> GPVEDAVTAAIGRVADTVGTGPTNSEAIPALTAAETGHTSQVVPGDTMQTRHVKNYHSRSESTVENFLCRSACVYFTEYKNSGSKRYAEWVVTTRQAAQLRRKLEFFTYIRFDLELTFVITSTQQPSTTQNQDAQILTHQIMYVPPGGPVPDKVDSYVWQTSTNPSVFWTEGNAPPRMSIPFLSIGNAYSNFYD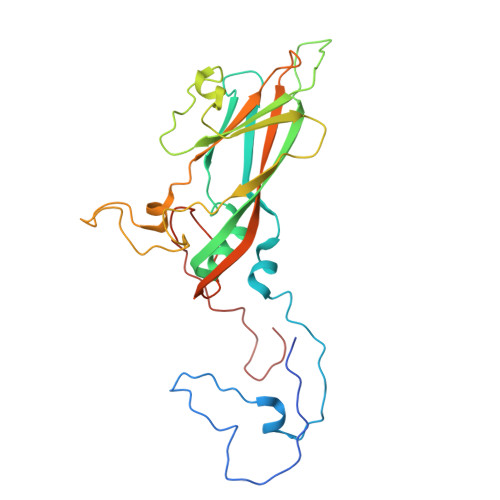GWSDFSRDGVYGINTLNSMGTLYARHVNTGGTGPIKSTIRIYFKPKHVKAWIPRPPRLCQYEKAKNVNFQPSGVTTTRQSITAMTNT> GSHMNGFTHYDVVIIGSGPAGSLCGIECRKKGLSVLCIEKEQFPRFHIGESLTGNAGQIIRDLGLAEDMDAAGFPDKPGVNVIGSLSKNEFFIPILAPTWQVRRSDFDDMIKRKAVEHGVEYKLGMVTDVIKDGEKVVGALYKADGVEHQVRSKVLVDASGQN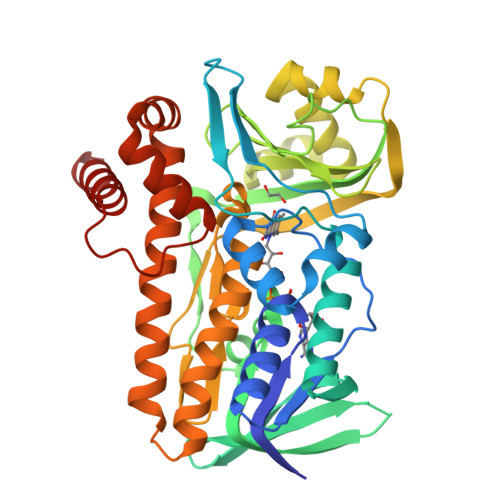TFLSRKGVAGKRQIEFFSQQIASFAHYKGVERDLPPFSTNTTILYSKQYHWSWIIPISPDTDSLGVVIPKDLYYKECKNPDDAIAWGMDHISPELKRRFKNAERQGDSQSMADFSYRIEPFVGDGWMCIGDAHRFLDPIFSYGVSFAMKEGIRAAEAIAQVVAGQDWKAPFYAYRDWSNGGQQIAADLIRYFWIYPIFFGYQMQNPDLRDEVIRLLGGCCFDCEGWKAPAIFRNAIEEYDRKQMAS Two crystal structures of recombinant Geobacillus stearothermophilus 6-phosphogluconate dehydrogenase (Gs6PDH) in complex with the substrate 6-­phosphogluconate have been determined at medium resolution. Gs6PDH shares significant sequence identity and structural similarity with the enzymes from Lactococcus lactis, sheep liver and the protozoan parasite Trypanosoma brucei, for which a range of structures have previously been reported. Comparisons indicate that amino-acid sequence conservation is more pronounced in the two domains that contribute to the architecture of the active site, namely the N-terminal and C-terminal domains, compared with the central domain, which is primarily involved in the subunit–subunit associations required to form a stable dimer. The high degree of structural similarity, efficient level of expression and straightforward crystallization conditions mean that Gs6PDH may prove to be an appropriate model system for structure-based inhibitor design targeting the enzyme from Trypanosoma species.

Two isomorphous crystal structures were determined. Data set I was obtained from a sample grown in the presence of 6PG and NADP+ and data set II was obtained from crystals grown in the presence of R5P and NADP+. In neither structure was there electron density that could be attributed to NADP+. However, structure II contained only 6PG, not R5P, and then only in one active site with a reduced occupancy of 0.7. This value was assigned following several rounds of refinement testing different levels of occupancy to elucidate that which gave clean difference density maps and thermal parameters consistent with the amino-acid side chains in the vicinity of the ligand. We have no definitive explanation of why we only see partially ordered 6PG in one active site of structure II, although we note a difference in the time that elapsed between crystal growth and cryo-freezing. The crystals used to generate data set II were frozen after a period of two months. The only significant difference is that structure II only has 6PG in a single active site and at a reduced occupancy. The overlay of 467 Cα positions of structure I subunit A on subunit B results in an r.m.s.d. of 0.53 Å; for structure II an r.m.s.d. of 0.70 Å is observed from the overlay of 470 Cα atoms. The overlay of the structure I and structure II dimers, 935 Cα atoms, gives an r.m.s.d. of 0.29 Å.

>GHMAKHQIGVIGLAVMGKNLALNIESKGYSVAVYNRLREKTDEFLQEAKGKNIVGTYSIEEFVNALEKPRKILLMVKAGAPTDATIEQLKPHLEKGDIVIDGGNTYFKDTQRRNKELAELGIHFIGTGVSGGEEGALKGPSIMPGGQKEAHELVRPIFEAIAAKVDGEPCTTYIGPDGAGHYVKMVHNGIEYGDMQLIAEAYFLLKHVLGMDAAELHEVFADWNKGELNSYLIEITADIFTKIDEETGKPLVDVILDKAGQKGTGKWTSQNALDLGVPLPIITESVFARFLSAMKDERVKASKVLAGPAVKPFEGDRAHFIEAVRRALYMSKICSYAQGFAQMKAASEEYNWNLRYGDIAMIFRGGCIIRAQFLQKIKEAYDRDPALSNLLLDSYFKDIVERYQDALREIVATAAMRGIPVPGSASALAYYDSYRTAVLPANLIQAQRDYFGAHTYERVDKEGIFHTEWLK[2x]> SNAETIEIIKDLFEHLCGVRVHRTYEDDTGLWFDTSQGSKNGIMDYKLGFVKSQAENTTEVDTEVIYVPLLKQRTAEELQELQKKLPDYLFETLSFPLRSLNQFYIKMSKSLNKKV;> SNAPTLGERLDSLHEIKSARRMDHFN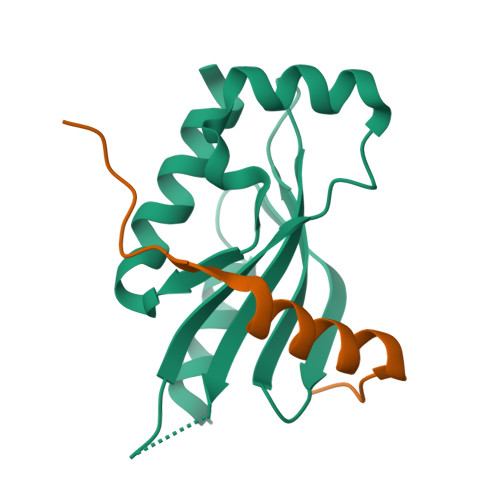DD>MADIYPLGKTHTEELNEIIVESAKEIAEPDTTMIQKLIDEHNPEPLLKGVRYYMCENDIEKKRRTYYDAAGQQLVDDTKTNNRTSHAWHKLFVDQKTQYLVGEPVTFTSDNKTLLEYVNELADDDFDDILNETVKNMSNKGIEYWHPFVDEEGEFDYVIFPAEEMIVVYKDNTRRDILFALRYYSYKGIMGEETQKAELYTDTHVYYYEKIDGVYQMDYSYGENNPRPHMTKGGQAIGWGRVPIIPFKNNEEMVSDLKFYKDLIDNYDSITSSTMDSFSDFQQIVYVLKNYDGENPKEFTANLRYHSVIKVSGDGGVDTLRAEIPVDSAAKELERIQDELYKSAQAVDNSPETIGGGATGPALEKLYALLDLKANMAERKIRAGLRLFFWFFAEYLRNTGKGDFNPDKELTMTFTRTRIQNDSEIVQSLVQGVTGGIMSKETAVARNPFVQDPEEELARIEEEMNQYAEMQGNLLDDEGGDDDLEEDDPNAGAAESGGAGQVS[2x];>[2x]MDIQRVKRLLSITNDKHDEYLTEMVPLLVEFAKDECHNPFIDKDGNESIPSGVLIFVAKAAQFYMTNAGLTGRSMDTVSYNFATEIPSTILKKLNPYRKMAR;>MYEEFRDVITFQSYVEQSNGEGGKTYKWVDEFTAAAHVQPISQEEYYKAQQLQTPIGYNIYTPYDDRIDKKMRVIYRGKIVTFIGDPVDLSGLQEITRIKGKEDGAYVG[2x];> MTWKLASRALQKATVENLESYQ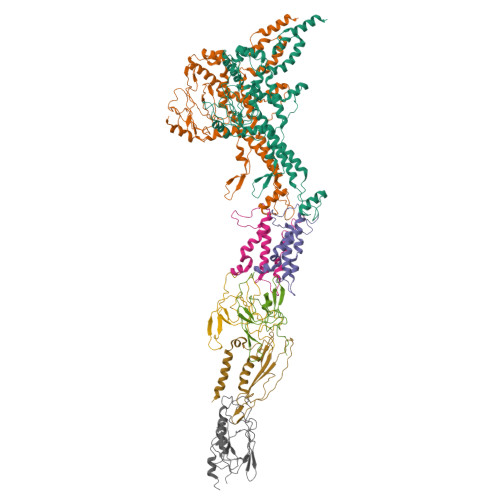PLMEMVNQVTESPGKDDPYPYVVIGDQSSTPFETKSSFGENITMDFHVWGGTTRAEAQDISSRVLEALTYKPLMFEGFTFVAKKLVLAQVITDTDGVTKHGIIKVRFTINNN;> MPETPIMGQDVKYLFQSIDAATGSAPLFPAYQTDGSVSGERELFDEQTKNGRILGPGSVADSGEVTYYGKRGDAGQKAIEDAYQNGKQIKFWRVDTVKNENDKYDAQFGFAYIESREYSDGVEGAVEISISLQVIGELKNGEIDTLPEEIVNVSKGGYDFQQPGQTTGEAPGTVPAP> MDKTHVLRNTTRGMFRTSMMRVLGRPGSLSVTASAGGTACVPMAALLRRSATPAAASATAASAMSALWCTRC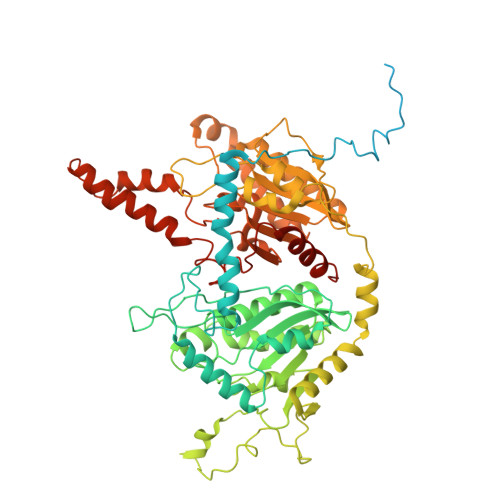FESSSAGSPPKVSDAGMKERSTQEPCVAATPTPSDTAATLAAAATPAPAAPIKSKGVDYARLYAHHPIDYERSTSKSPNILRLPANTSDPTYQENMARMEGLVEQLRARVRYVQAGGVVPEEEAAKAGVSISSIEADDRVRKLHLSRGKMLARDRIERLIDPGTRFLELSQLAGWDLYWDDKKKEYERCYSGGIVTGIGLVNGVRCMLVANDATVKGGTYYPITVKKHLRAQKIAEQNHLPCIYLVDSGGANLSRQDDVFPDEQHFGRIFYNEAQMSIKSISQIAVVMGSCTAGGAYVPAMADENIIVARNGTIFLGGPPLVLAATGEKVSSEELGGADVHCRISGVGDHYATDDLHALYLARRAVANLNLKEHNEARNPTDVKPVPPLYDPRELGGFIPDMLSDVVKSFDVRAIIARIVDGSRFDEFKALYGNTLVCGFARIEGMQVGIIANQGILYSESALKGAHFIGLCTQRNVPLLFLQNITGFMVGKKYEEGGIARNGARLVMAVSSAPVPKVTVLIGGSYGAGNYGMCGRAFEPRFLFMWPNARISVMGGTQAATVLTLTNRNLKNASEAEIAAFKDKVKKKYEKEGSCYYSTARLWDDGVIAPEDTRVVVAEALRATRLAPMEKRERV> S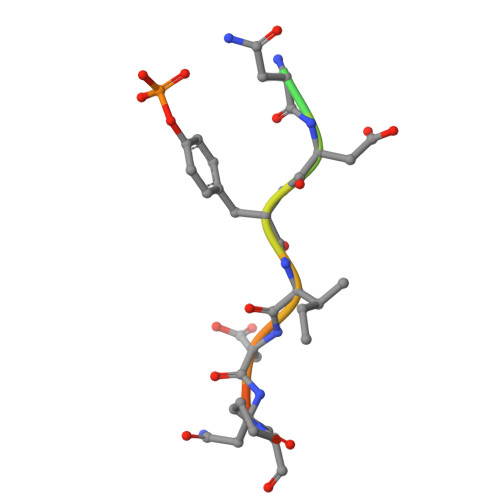HVENDYIDNPSL>[2x]MGSSHHHHHHSQDPAVPYNRMKLMIVGNTGSGKTTLLQQLMKTKKSDLGMQSATVGIDVKDWPIQIRDKRKRDLVLNVWDFAGHEEFYSTHPHFMTQRALYLAVYDLSKGQAEVDA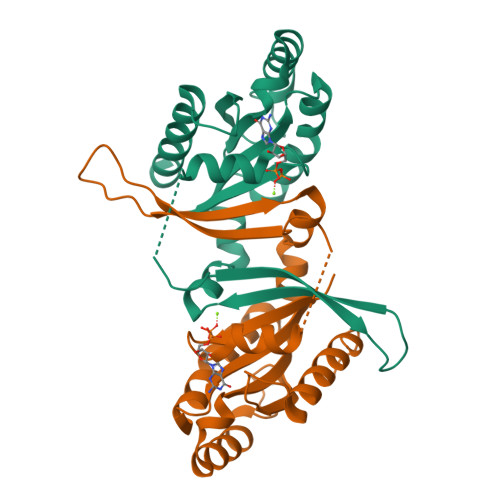MKPWLFNIKARASSSPVILVGTHLDVSDEAQRAACMSKITKELLNKRGFPAIRDYHFVNATEESDALAKLRKTIINESLNFKIRDQLVVG> MFENITTAPADPILGLADLLRADER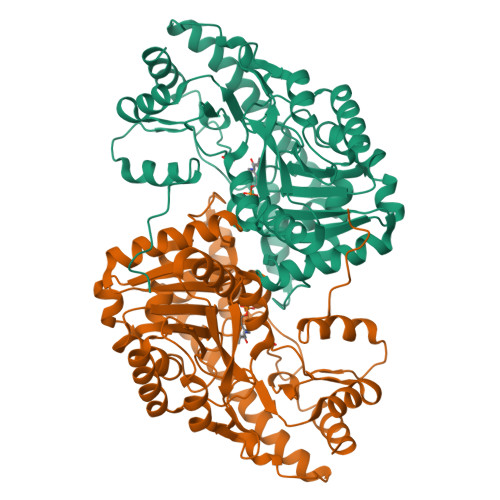PGKIDLGMGVYNDETGKTPVLTSVKKAEQYLLENETTKNYLGIDGIPEFGRCTQELLFGKGSALINDKRARTAQTPGGTGALRVAADFLAKNTSVKRVWVSNPGWPTHKSVFNSAGLEVREYAYYDAENHTLDFDALINSLNEAQAGDVVLFHGCCHNPTGIDPTLEQWQTLAQLSVEKGWLPLFDFAYQGFARGLEEDAEGLRAFAAMHKELIVASSYSKNFGLYNERVGACTLVAADSETVDRAFSQMKAAIRVNYSSPPAHGASVVATILSNDALRAIWEQELTDMRQRIQRMRQLFVNTLQEKGANRDFSFIIKQNGMFSFSGLTKEQVLRLREEFGVYAVASGRVNVAGMTPDNMAPLCEAIVAVL> GSHMSTPARRRLMRDFKRLQEDPPAGVSGAPSENNIMVWNAVIFGPEGTPFEDGTFKLTIEFTEE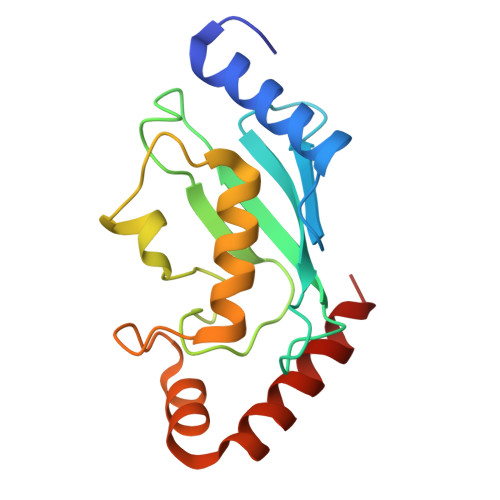YPNKPPTVRFVSKMFHPNVYADGSICLDILQNRWSPTYDVSSILTSIQSLLDEPNPNSPANSQAAQLYQENKREYEKRVSAIVEQSWRDC>MYMSKYVPVYTLLILIYSFNASAEWTGDKTNAYYSDEVISELHVGQIDTSPYFCIKTVKANGSGTPVVACAVSKQSIWAPSFKEL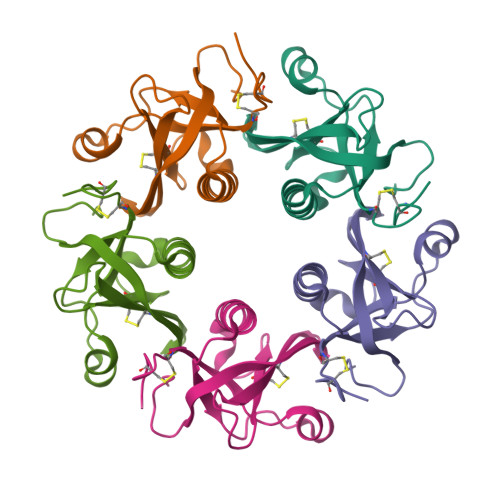LDQARYFYSTGQSVRIHVQKNIWTYPLFVNTFSANALVGLSSCSATQCFGPKLEHHHHHH[5x]> MNLPTAQEVQGLMARYIELVDVGDIEAIVQMYADDATVEDPFGQPPIHGREQIAAFFRQGLGGGKVRACLTGPVRASHNGCGAMPFRVEMVWNGQPCALDVIDVM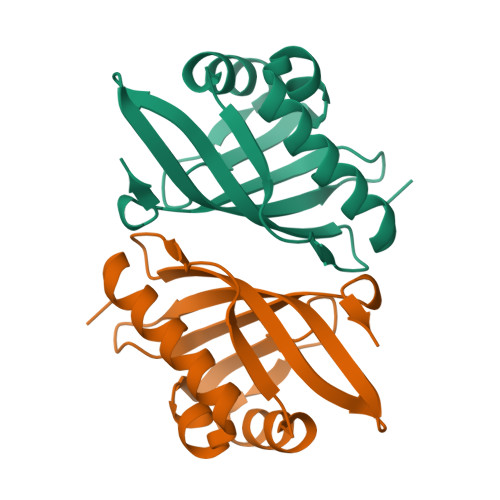RFDEHGRIQTMQAYWSEVNLSVREPQ>[2x]QVINTFDGVADYLQTYHKLPDNYITKSEAQALGWVASKGNLADVAPGKSIGGDIFSNREGKLPGK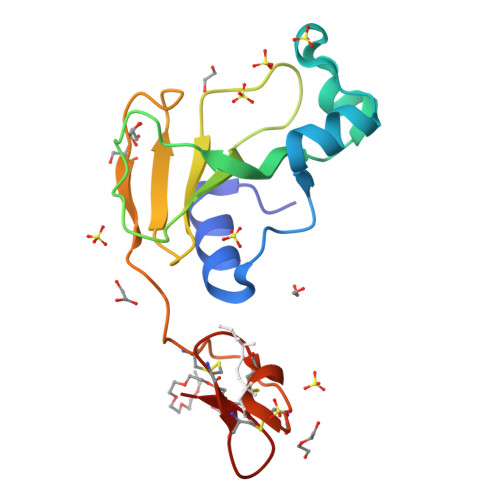SGRTWREADINYTSGFRNSDRILYSSDWLIYKTTDAYQTFTKIRSSSMGVCPKILKKCRRDSDCLAGCVCGPNGFCGS> GAMGSAEAWYNLGNAYYKQGDYDEAIEYYQKALELDPRSAEAWYNLGNAYYKQGDYDEAIEYYQKALELDPRSAEAWYNLGNAY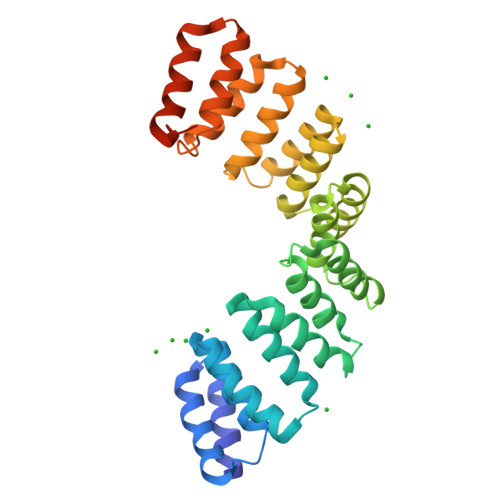YKQGDYDEAIEYYQKALELDPRSAEAWYNLGNAYYKQGDYDEAIEYYQKALELDPRSAEAWYNLGNAYYKQGDYDEAIEYYQKALELDPRSAEAWYNLGNAYYKQGDYDEAIEYYQKALELDPRSAEAWYNLGNAYYKQGDYDEAIEYYQKALELDPRSAEAWYNLGNAYYKQGDYDEAIEYYQKALELDPRSAEAKGNLGNAKQKQG>[4x]HHHHHHSSGENLYFQGMQTDSNPHDLAVAGILEQLEGCLRASDSTGAAQLFEPDGYWRDLVLFTWNLKTLEGREQIAAMLAAQLGAVQPVSIRIADGEHAVEAGGVLQSWITVETNVARGVGFIRIRDGKIWTLLTTMSELKGFEEAKGGRRPMGAEHGARTDRSSWLEQREQEAKELGYARQPYCVIIGGGQG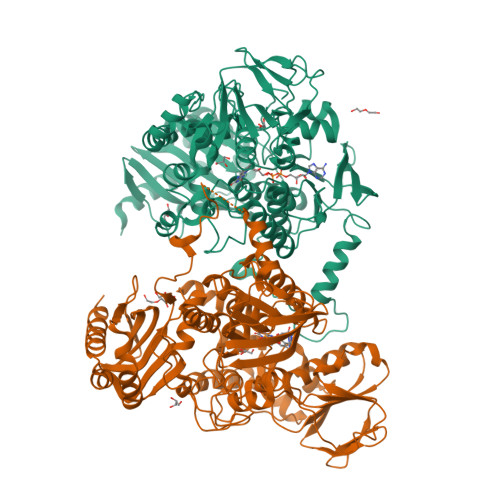GIALGARLRQLNVPTIIIEKNARPGDSWRKRYKSLCLHDPVWYDHMPYIPFPDNWPVFTPKDKVGDWLEMYTKVMELNYWGSTSCESASFDAASGEWTVQVLRDGQPVTLKPKQLVLATGMSGKANMPKFKGMDVFQGEQQHSSQHPGPDAYAGKKVVVVGANNSAHDICAALWEAGVDVTMVQRSSTHIVKSDSLMDLALGDLYSERALAAGMTTNKADLTFASIPYKILANFQKPVFKAIRERDADFYARLEERGFMLDFGDDDSGLFMKYLRRGSGYYIDVGASELVAEGKIKLKSGVGVQELKSHSIVLSDGTELPADLVVYATGYGSMNGWAADLISPEVANKVGKVWGLGSATTKDPGPWEGEQRNMWKPTQQQALWFHGGNLHQSRHYSQYLSLQLKARMEGLNTPVYGQQEVHHLS>[2x]GSIGAASMEFCFDVFKELKVHHANENIF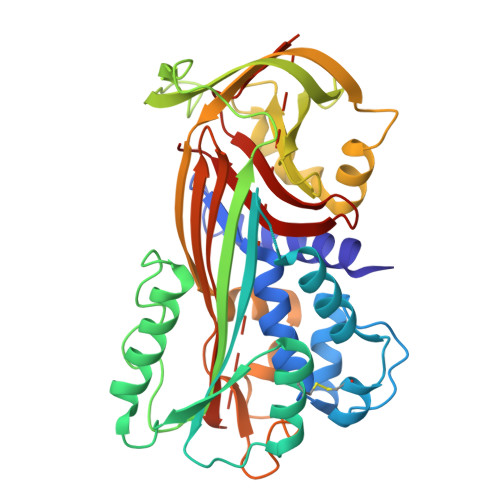YCPIAIMSALAMVYLGAKDSTRTQINKVVRFDKLPGFGDSIEAQCGTSVNVHSSLRDILNQITKPNDVYSFSLASRLYAEERYPILPEYLQCVKELYRGGLEPINFQTAADQARELINSWVESQTNGIIRNVLQPSSVDSQTAMVLVNAIVFKGLWEKTFKDEDTQAMPFRVTEQESKPVQMMYQIGLFRVASMASEKMKILELPFASGTMSMLVLLPDEVSGLEQLESIINFEKLTEWTSSNVMEERKIKVYLPRMKMEEKYNLTSVLMAMGITDVFSSSANLSGISSAESLKISQAVHAAHAEINEAGTEVVGSAEAGVDAASVSEEFRADHPFLFCIKHIATNAVLFFGRCVSP> STLYEKLGGTTAVDLAVDKFYERVLQDDRIKHFFADVDMAKQRAHQKAFLTYAFGGTDKYDGRYMREAHKELVE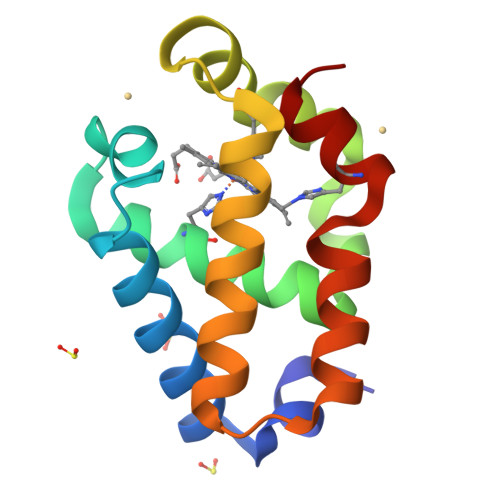NHGLNGEHFDAVAEDLLATLKEMGVPEDLIAEVAAVAGAPAHKRDVLNQ>[12x]MINVDGEYLKIFAGRIKLMKAVILAAGLGTRLGGVPKPLVRVGGCEIILRTMKLLSPHVSEFIIVASRYADDIDAFLKDKGFNYKIVRHDRPEKGNGYS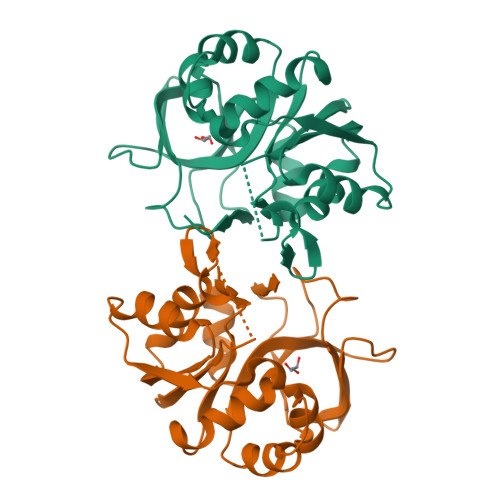LLVAKNHVEDRFILTMGDHVYSQQFIEKAVRGEGVIADREPRFVDIGEATKIRVEDGRVAKIGKDLREFDCVDTGFFVLDDSIFEHAEKLRDREEIPLSEIVKLARLPVTYVDGELWMDVDTKEDVRRANRAL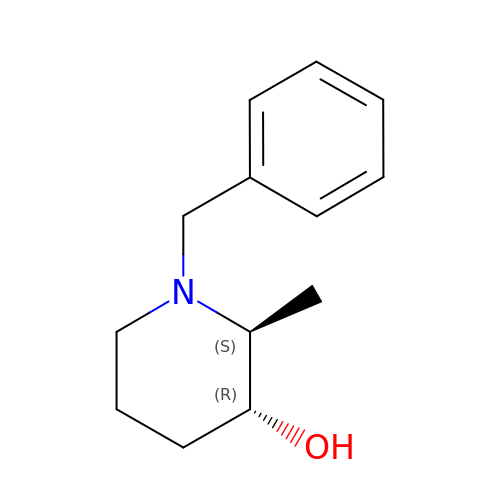(2S,3R)-1-benzyl-2-methylpiperidin-3-ol | C13 H19 N O | ZFJGRVQFTNBLRP-UHFFFAOYSA-N~{N}-[4-[(3~{a}~{S},4~{S},6~{a}~{R})-2-oxidanylidene-1,3,3~{a},4,6,6~{a}-hexahydrothieno[3,4-d]imidazol-4-yl]butyl]-9,10-bis(oxidanylidene)anthracene-2-carboxamide 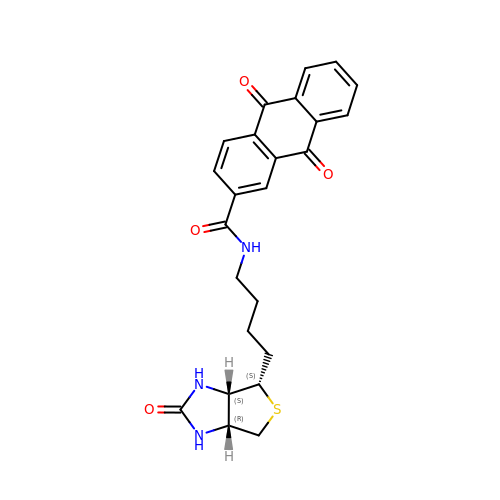| C24 H23 N3 O4 S | ISFDLFAYCAKKAR-UFYCRDLUSA-N>DYKDDDDKRPHLEVALLRDDFRQNPTDVVVAAGEPAILECQPPRGHPEPTIYWKKDKVRIDDKEERISIRGGKLMISNTRKSDAGMYTCVGTNMVGERDSDPAELTVFERPTFLRRPINQVVLEEEAVEFRCQVQGD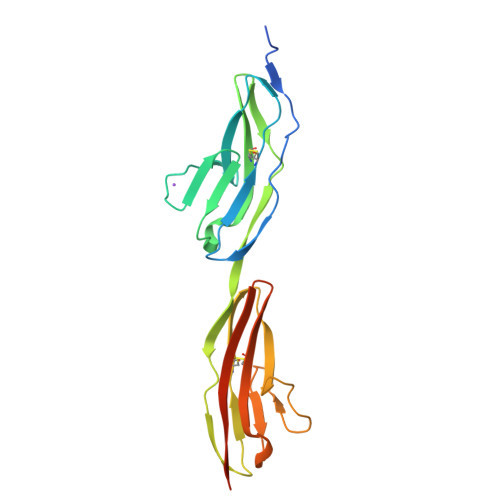PQPTVRWKKDDADLPRGRYDIKDDYTLRIKKTMSTDEGTYMCIAENRVGKMEASATLTVRAKLGSHHHHHH[2x]>[3x]QGAVRKATAAEIAALPRQKVELVDPPFVHAHSQVAEGGPKVVEFTMVIEEKKIVIDDAGTEVHAMAFNGTVPGPLMVVHQDDYLELTLINPETNTLMHNIDFHAATGALGGGGLTEINPGEKTILRFKATKPGVFVYHCAPPGMVPWHVVSGMNGAIMVLPREGLHDGKGKALTYDKIYYVGEQDFYVPRDENGKYKKYEAPGDAYEDTVKVMRTLTPT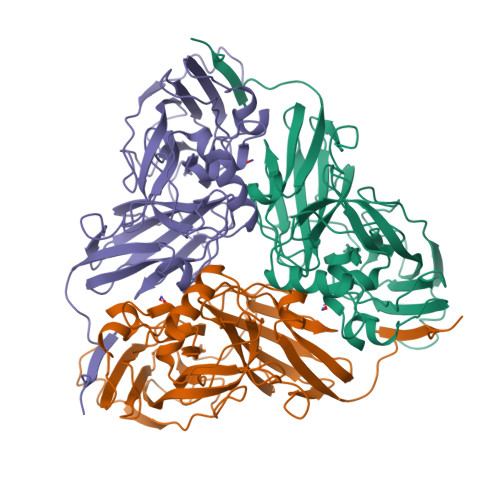HVVFNGAVGALTGDKAMTAAVGEKVLIVHSQANRDTRPHLIGGHGDYVWATGKFNTPPDVDQETWFIPGGAAGAAFYTFQQPGIYAYVNHNLIEAFELGAAAHFKVTGEWNDDLMTSVLAPSGT> MSEGKLEKLRIVAYKDSKFSDEVENGEFITLLNPEKYKFQYRVEQNEDQASGTSSAPIRFNKILPQTLEFDFLFDRTGVIAGYEVTEDGIINDIDHFKKVVYDYNGEKHKPNYLMITWGSLLFKGYLKEMDIEYKLFRPDGTPIRAMATTKIGEFVEEELRTAQENNQSPDMSHYRTVKEGDTLPLMTYRIYGDSKYYLEVAKANGLTNF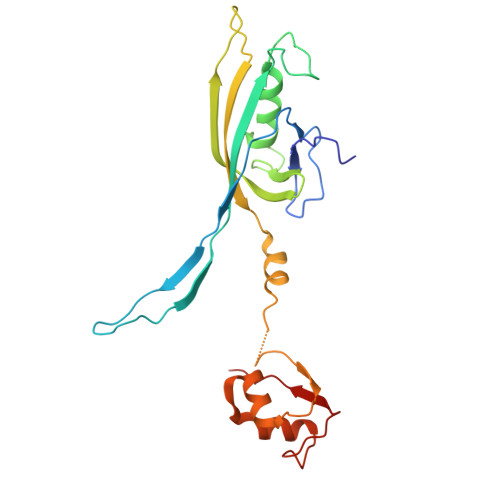RRLKTGTELIFPPLQKQK> SNAMVSNSNVNLQKIFDENKITGSVTIYDYKNKIWIYSNEEDSKIRRLPASTFKIPNSLIFLEEEVVKDENEAMEWDGIKRYIENWNKDLNLREAYEYSALWFYMKGAGKIKSEKYKEYLKEFNYGNQIVSEKKNSFWIDRSLKISPEEQIDFLINLYEEKFMLSEKTYKIVKDIMINEKTPEYTLRGKTGWGREGAENIIWYVGY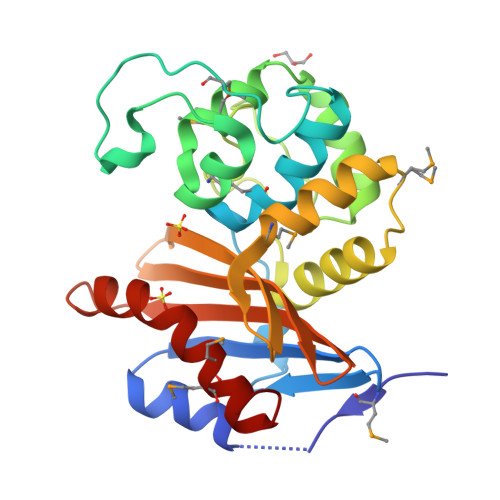IEAKENVYFFAVRIINASEERNSYLLDFRKQLTMMAFRELGIIN>GHMNLSQLSFHRVDQKEITQLSHLGQGTRTNVYEGRLRVEGSGDPEEGKMDDEDPLVPGRDRGQELRVVLKVLDPSHHDIALAFYETASLMSQVSHTHLAFVHGVCVRGPENIMVTEYVEHGPLDVWLRRERGHVPMAWKMVVAQQLASALSYLENKNLVHGNVCGRNILLARLGLAEGTSPFIKLSDPGVGLGALSREERVERIPWLAPECLPGGANSLSTAMDKWGFGATLLEICFDGEAPLQSRS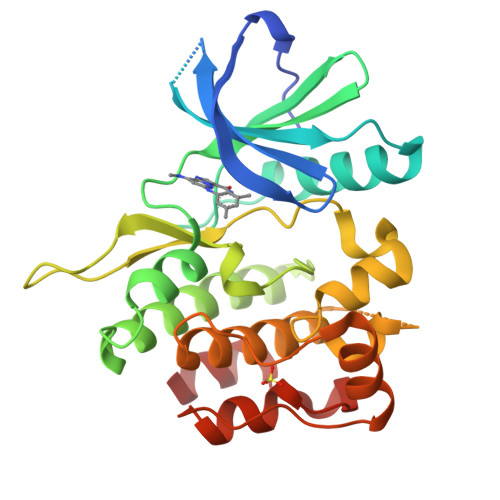PSEKEHFYQRQHRLPEPSCPQLATLTSQCLTYEPTQRPSFRTILRDLTRL[2x]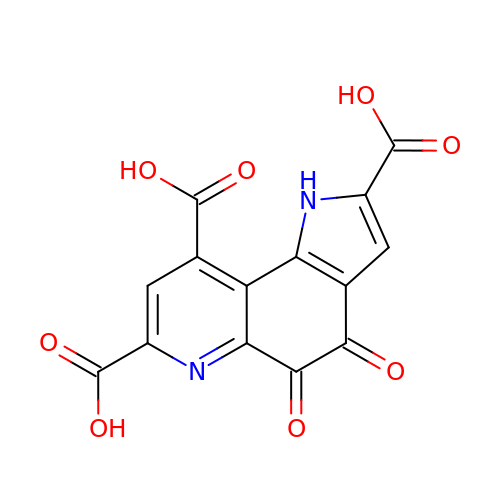PYRROLOQUINOLINE QUINONE | C14 H6 N2 O8 | MMXZSJMASHPLLR-UHFFFAOYSA-N>AMGRDSLINSMVEGVLGINESRQIILSNKMANDIMDNIDEDAKAFLLRQIEDTFKSKQTEMRDLEMNTRFFVVTTSYIDKIEQGGKSGVVVTVRDMTNEHNLDQ[2x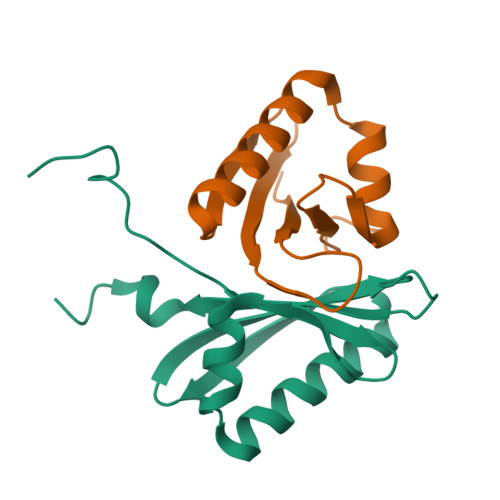]Responding to this critical need, we introduce here a fully automated method for collecting, selecting, and merging data from hundreds to thousands of in meso-grown microcrystals. This approach boosts the collective phasing signal of many tiny crystals to a level where de novo phasing of highly challenging membrane protein targets becomes not only possible but also fast and high-throughput. We refer to it as the in meso in situ serial crystallography—experimental phasing (IMISX-EP) method. IMISX-EP has three components: (1) in meso crystallization (and in situ soaking where appropriate), (2) fast, automated grid scanning, and serial data collection in situ, and (3) real-time data processing and selection of data sets followed by structure solution.

We demonstrated the IMISX-EP approach for both heavy atom derivatization methods with two membrane proteins, BacA and PgpB. Indeed, BacA is the first de novo structure solved by the IMISX-EP method. BacA crystals were derivatized by in situ soaking with HgCl2 in IMISX wells directly. From the 968 BacA crystals identified, two groups were created with which to evaluate two phasing methods. One contained 360, the other 271 data sets. The first group was used successfully for SAD phasing with SHELXD and CRANK2. Another advantage is the ease with which heavy atom and ligand-soaking experiments can be performed in true in situ fashion without ever touching the crystals, which remain suspended in the viscous mesophase.

> MHHHHHHGSMSDMHSLLIAAILGVVEGLTEFLPVSSTGHMIIVGHLLGFEGDTAKTFEVVIQLGSILAVVVMFWRRLFGLIGIHFGRPLQHEGESKGRLTLIHILLGMIPAVVLGLLFHDTIKSLFNPINVMYALVVGGLLLIAAECLKPKEPRAPGLDDMTYRQAFMIGCFQCLALWPGFSRSGATISGGMLMGVSRYAASEFSFLLAVPMMMGATALDLYKSWGFLTSGDIPMFAVGFITAFVVALIAIKTFLQLIKRISFIPFAIYRFIVAAAVYVVFF> GAMGDVSRLNQRNINELKIFVEKAKYYSIKLDAIYNECTGAYNDIMTYSEGTFSDQSKVNQAISIFKKDNKIVNKFKELEKIIEEY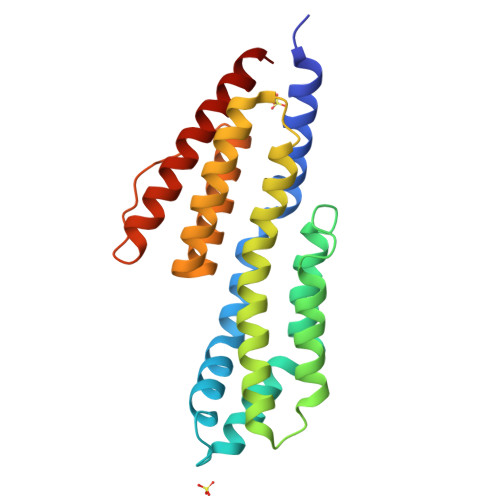KPMFLSKLIDDFAIELDQAVDNDVSNARHVADSYKKLRKSVVLAYIESFDVISSKFVDSKFVEASKKFVNKAKEFVEENDLIALESIVKTIGDMVNDREINSRSRANNFAKKEADFLGAAVELEGAYKAIKQTLL>[2x]GCTGNFEDYNKNPHEPDQNDMGVDWYLVRSLALNLQDLMMPEQENFSQYVDCLMAGAFSGYVADSNLGTGWSGRYATYNPSDDWKKIPFNDFYSKFYPDYFNLKNQSDDELFLSLAELYRIVVMLRVTDTYGPIPYSKVGAANAIKSPYDSQQAVYAKMLEDLDNIITVLGKFGNQSFSSSADRIYNGNTSAWYKFANSLKLRMAMRTCYVAGFNVNGKTSQQLAEEAVAAGVMTAATDGAYRKVADHNPWQRFMVLWSDARISADLTCYMNAYNDPRREAYYDKSTFGTVSGNAYTGEESYVGLRRGILQGQYNSWSQGSSCMKVTTSDNIVVFRASEVAFLRAEGALRNWNMGGTAKDFYEEGIRLSFEENGITSGVENYLASTGKVEAYKDPLKGQSAQTYDYSGAINTNVTVAWSGGDFEKSLEQIITQKWIANFPNGMESWTE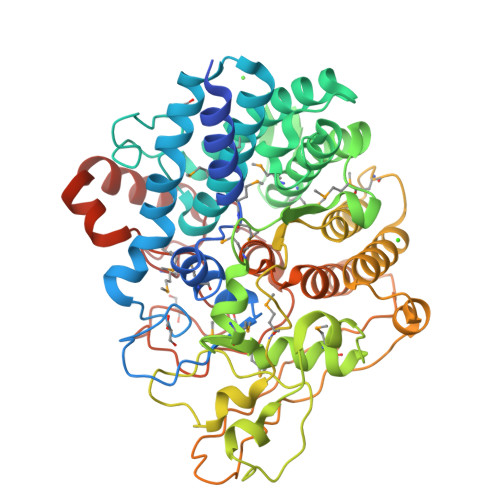YRRTGYPKLMPMAANASGGIVNDAEGARRMPYPTDEYRENRESVEAAVATLTQESKTKRGDTMATHVWWDCK>MAHHHHHHMIYPNILATIGHTPVVKINRLGKDLECEL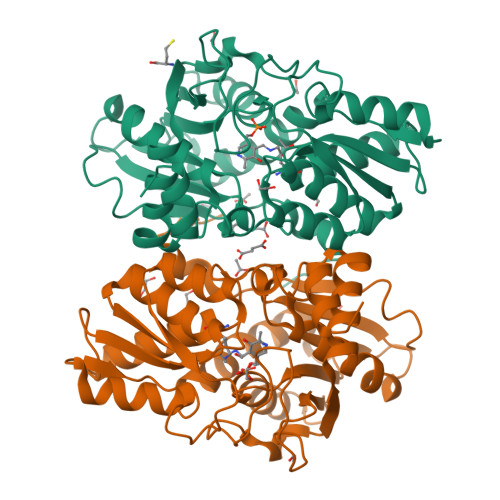YAKCEFFNPGGSVKDRIGYEMVVKAEKEGRIKPGDTLIEPTSGNTGIGIALAGAVLGYKVIITMPEKMSQEKQSVLERLGAIIYRTPTEAAYNDPDSHISLAKKLQAEIPNSHILDQYANPNNPNAHYFGTAQEIIDDFGKDLHMVVAGVGTGGTITGIAKRLKEFNPAIKIIGADPEGSILGGGTEIKSYHVEGIGYDFFPDVLDNTLIDAYIKTNDADSFRTARRLIKEEGLLIGGSCGAAMWAALQAAKSLSKGQKCLVILPDSIRNYMSKFANDEWMKEMGFL[2x]> MAHHHHHHVDDDDKDLFNKNKKLDADLLKTLDNLLKTLDN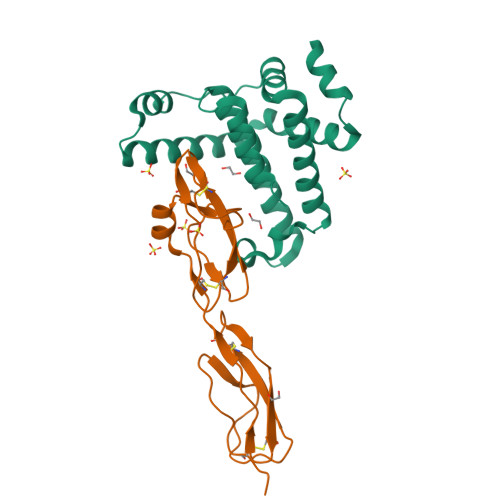NQKQALIYFKDKLQDKKYLNDLMEQQKSFLDNLQKKKEDPDLQDRLKKTLNSEYDESQFNKLLNELGNAKAKQFLQQLHIMLQSIKDGTLTSFSSSNFNDLQNLEQKKERALQYINGKLYVEYYFYINGISNADNFFETIMEYLKT;> AGIQNDSTGKCGPPPPIDNGDITSFPLSVYAPASSVEYQCQNLYQLEGNKRITCRNGQWSEPPKCLHPCVISREIMENYNIALRWTAKQKLYSRTGESVEFVCKRGYRLSSRSHTLRTTCWDGKLEYPTCAKR> GPLGSQKVEKKIRAKAFQKCPICEKVIQGAGKLPRHIRTHTGEKPYECNICKVRFTRQDKLKVHMRKHTGEKPYLCQQCGAAFAHNYDLKNHMRVHTGLRPYQCDSCCKTFVR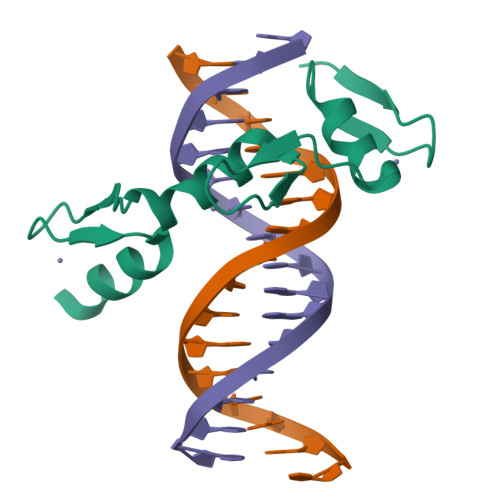SDHLHRHLKKDGCNGVPSRRGRKLERPHRD> MTHQIVTTQYGKVKGTTENGVHKWKGIPYAKPPVGQWRFKAPEPPEVWEDVLDATVYGPVCPQPSDLLSLSYKELPRQSEDCLYVNVFAPDTPSQNLPVMVWIHGGAFYLGAGSE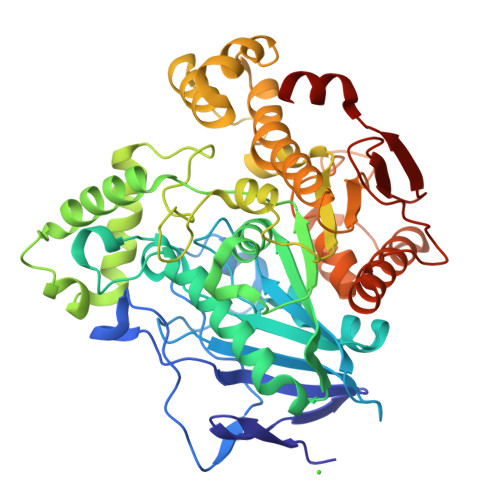PLYDGSKLAAQGEVIVVTLNYRLGPFGFMHLSSFDEAYSDNLGLLDQAAALKWVRENISAFGGDPDNVTVFGESAGGMSIAALLAMPAAKGLFQKAIMESGASRTMTKEQAASTAAAFLQVLGINESQLDRLHTVAAEDLLKAADQLRIAEKENIFQLFFQPALDPKTLPEEPEKSIAEGAASGIPLLIGTTRDEGYFFFTPDSDVYSQETLDAALEYLLGKPLAEKVADLYPRSLESQIHMVTDLLFWRPAVAFASAQSHYAPVWMYRFDWHPEKPPYNKAFHTLELPFVFGNLDELERMAKAEITDEVKQLSHTIQSAWTTFAKTGNPSTEAVNWPAYHEESRETVILDSEITIENDPESEKRQKLFPSKGE>[4x]MTKDQNGTWEMESNENFEGYMKALDIDFATRKIAVRLTQTKI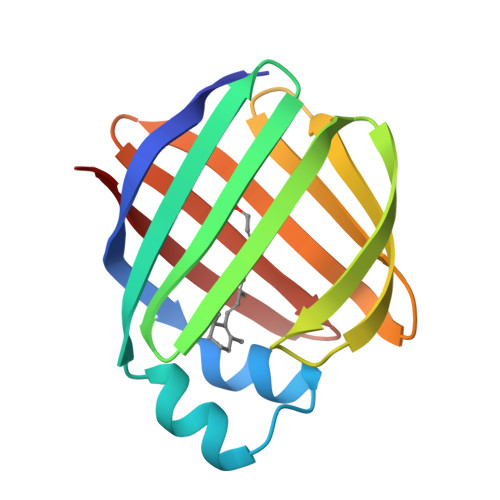IVQDGDNFKTKTNSTFRNYDLDFTVGVEFDEHTKGLDGRNVKTLVTWEGNTLVCVQKGEKENRGWKQWVEGDKLYLELTCGDQVCRQVFKKK>MDLTVEPNLHSLITSTTHKWIFVGGKGGVGKTTSSCSIAIQMALSQPNKQFLLISTDPAHNLSDAFGEKFGKDARKVTGMNNLSCMEIDPSAALKDMNDMAVSRANNNGSDGQGDDLGSLLQGGALADLTGSIPGIDEALSFMEVMKHIKRQEQDEGETFDTVIFDTAPTGHTLRFLQLPNTLSKLLEKFGEITNKLGPMLNSFMGAGNVDISGKLNELKANVETIRQQFTDPDLTTFVCVCISEFLSLYETERLIQELISYDMDVNSIIVNQLLFAENDQEHNCKRCQARWKMQKKYLDQIDELYEDFHVVKMPLC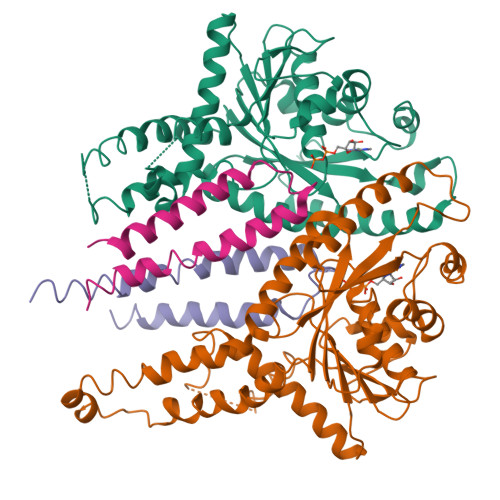AGEIRGLNNLTKFSQFLNKEYNPITDGKVIYELEDKELEHHHHHH[4x];>TNKYHEKWISKFAPGNELSKKYLAKVKERHELKEFNNSISAQDNYAKWTKNNRKLDSLDKEINNLKDEIQSENKAFQAHLHKLR[4x]>MKTERENGIVRQVNTIQTKEERFNPFSWYEEMRNTAPVQWDEERQVWDVFHYDGVKEVLEQKNIFSSDRRPPQNQRQTALGTSLINIDPPKHAEMRALVNKAFTPKAMKAWEPKIARITNELLQEVEHLEDIDIVEHLSYPLPVMVIADILGVPIEDQRQFKDWSDIIVAGPSNNERETLEKLQQEKMKANDELETYFYRIIEEKRTRPGDDIISVLLQAKEEGKQLTDEEIVGFSILLLIAGNETTTNLISNTIYCLMEDKASFERLKREKELLPSGIEEVLRYRSPVQALHRIVKEDVTLAGKKLKAGEHVVPWMGSAHRDAEYFEDPEVFKIDRKPNVHMAFGRGIHFCLGAPLARIEAKIMLAELIDRYPQMDWSPSFELKPIESTFVY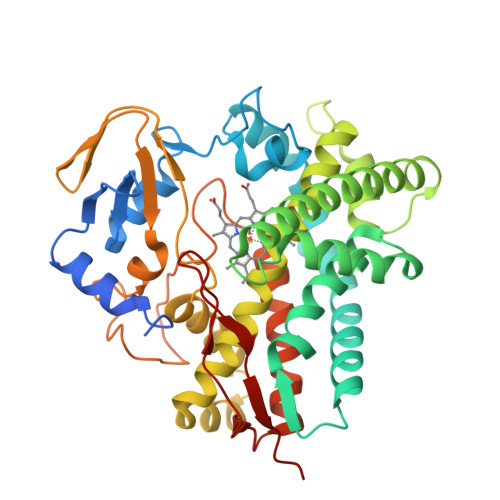GLKELLIRKNVHHHHHH[2x]> ALKPLKTWSHLAGNRRRPSEYEVVSTNLHYFTDNPERPWELDSNLPMQTWYKKYCFDSPLKHDDWNAFRDPDQLVYRTYNLLQDGQESYVQGLF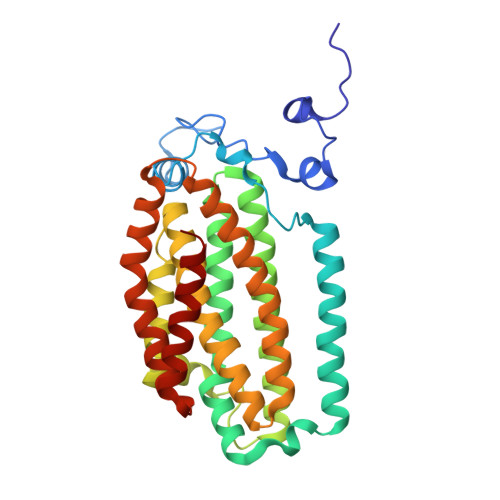DQLNDRGHDQMLTREWVETLARFYTPARYLFHALQMGSVYIHQIAPASTITNCATYETADHLRWLTHTAYRTRELANCYPDVGFGKRERDVWENDPAWQGFRELIEKALIAWDWGEAFTAINLVTKPAVEEALLQQLGSLAQSEGDTLLGLLAQAQKRDAERHRRWSSALVKMALEKEGNREVLQKWVAKWEPLADKAIEAYCSALPDGENAIVEAKSASRYVRQMMG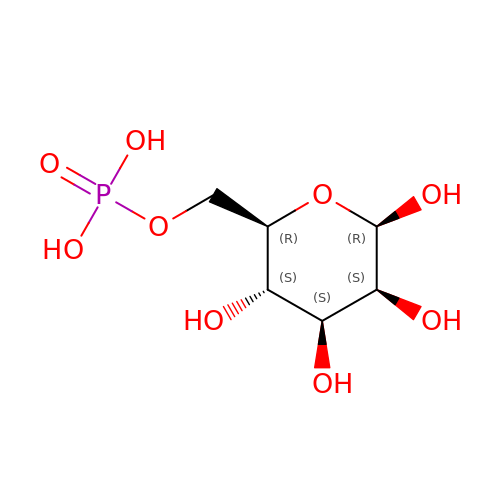6-O-phosphono-beta-D-mannopyranose | C6 H13 O9 P | NBSCHQHZLSJFNQ-RWOPYEJCSA-N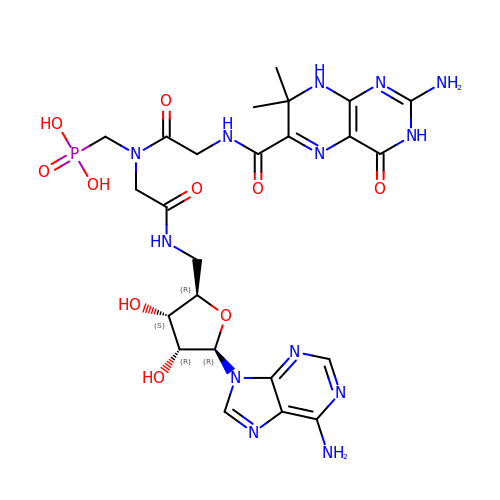((2-(2-amino-7,7-dimethyl-4-oxo-3,4,7,8-tetrahydropteridine-6-carboxamido)-N-(2-((((2R,3S,4R,5R)-5-(6-amino-9H-purin-9-yl)-3,4-dihydroxytetrahydrofuran-2-yl)methyl)amino)-2-oxoethyl)acetamido)methyl)phosphonic acid | C24 H32 N13 O10 P | IHZBIHWJVSGIOO-MDNHXVGFSA-N> MNTVPFTSAPIEVTIGIDQYSFNVKENQPFHGIKDIPIGHVHVIHFQHADNSSMRYGYWFDCRMGNFYIQYDPKDGLYKMMEERDGAKFENIVHNFKERQMMVSYPKIDEDDTWYNLTEFVQMDKIRKIVRKDENQFSYVDSSMTTVQENELLKSSLQKAGSKMEAKNEDDPAHSLNYTVINFKSREAIRPGHEMEDFLDKSYYLNTVMLQGIFKNSSNYFGELQFAFLNAMF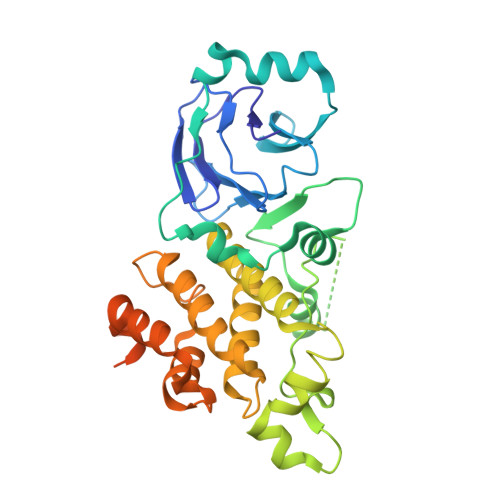FGNYGSSLQWHAMIELICSSATVPKHMLDKLDEILYYQIKTLPEQYSDILLNERVWNICLYSSFQKNSLHNTEKIMENKYPELLGKDNEDDALIYGISDEERDDEDDEHNPTIVGGLYYQRPLEHHHHHH N-[(1R,3R)-3-hydroxy-1-(hydroxymethyl)-3-phenylpropyl]hexadecanamide 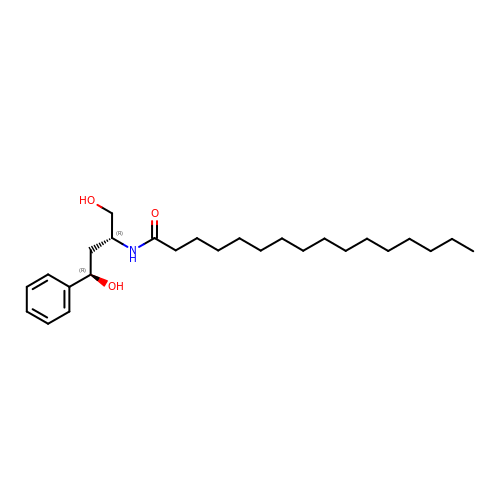| C26 H45 N O3 | BDMBWENRFFKJON-JWQCQUIFSA-N>[4x]MDNYQELAIQFAAQAVDRNEIEQWVREFAYQGFDARR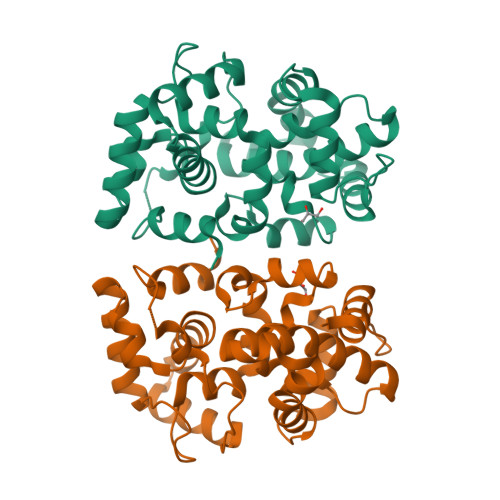VIELLKQYGGADWEKDAKKMIVLALTRGNKPRRMMMKMSKEGKATVEALINKYKLKEGNPSRDELTLSRVAAALAGRTCQALVVLSEWLPVTGTTMDGLSPAYPRHMMHPSFAGMVDPSLPGDYLRAILDAHSLYLLQFSRVINPNLRGRTKEEVAATFTQPMNAAVNSNFISHEKRREFLKAFGLVDSNGKPSAAVMAAAQAYKTAA>MMLKSVTESFAGMIHGLKVNHLTDGIIRRSKRMILDSLGVGFLGTGTEVFHKVTQYSKIYSSNTSSTVWGRPDFRLPPTYAAFVNGVAVHSMDFDDTWHPATHPSGAVLPVLTALSEALPQTPKFSGLDLLLAFNVGIEVQGRLMHFSKEAKDIPKRFHPPSVVGTLGSAAAASKFLGLSLTKCREALAIAVSHAGAPIANAATQTKPLHIGNAAKHGMEATFLAMLGLQGNKQILDLGSGFGAFYANYSPEDLPSLDSHIWLLDQQDVAFKSFPAHLATHWVADAAAAVRKHLVTPERALFPADHIERIVLRIPDVQYVNRPFPDSEHEARHSFQYVACASLLDGSITVPSFHSQQVNRPQVRELLKKVKLEHPPDNPPSFDTLYCEISITLKDGTTFTERSDTFYGHWRKPLSQEDLRNKFRANASKMLCRDTVESL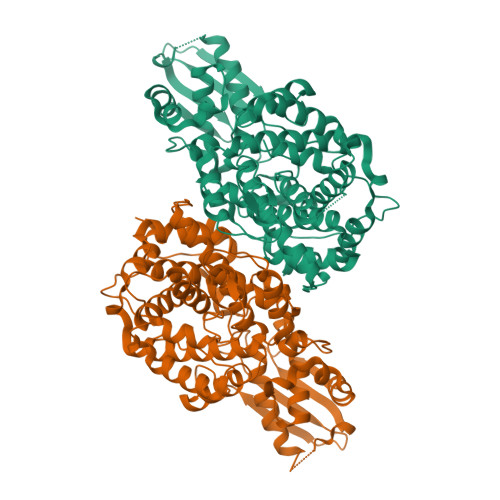ITVVEKLEDLEDCSVLTRLLKGPSVQDEASKLSSMSSFDHTTLPRFTNI[2x]>[4x]SPPQKVCLICGDEASGCHYGVLTCGSCKVFFKRAVEGQHNY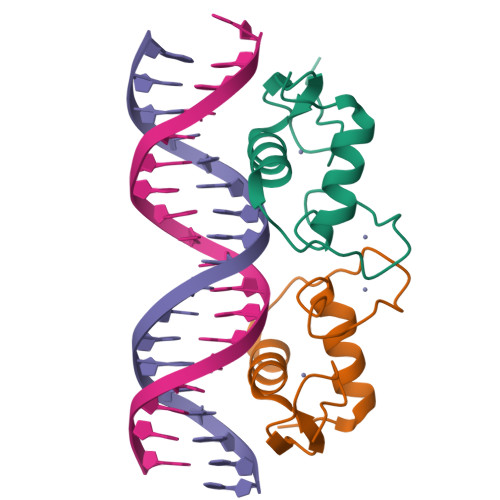LCAGRNDCIIDKIRRKNCPACRLRKCLQAGMTLGARKSKKL> MDLEKNYPTPRTSRTGHGGVNQLGGVFVNGRPLPDVVRQRIVELAHQGVRPCDISRQLRVSHGCVSKILGRYYETGSIKPGVIGGSKPK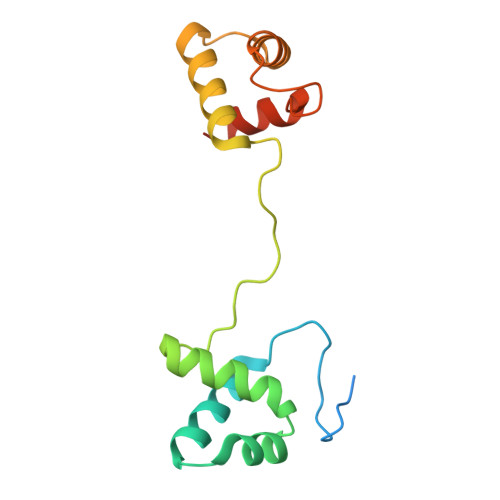VATPKVVEKIAEYKRQNPTMFAWEIRDRLLAERVCDNDTVPSVSSINRIIRTKVQQPPNQ>GPMAVPFSNTHLRIPRGFGNLLEGLTREVL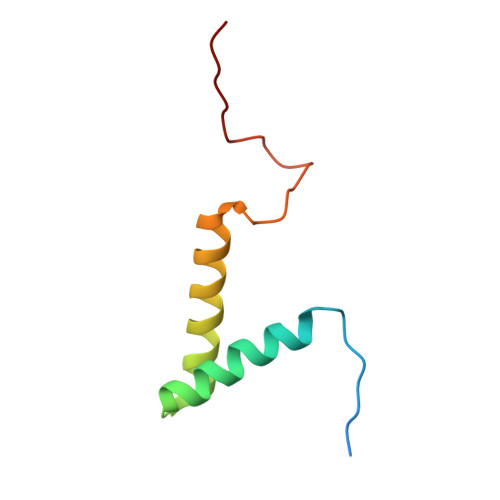REQPEDIATFAAVYFTELLKAREESGLDPAEWGAKLEDRFYNNH[4x]> TTFTTRDGTQIYYKDWGSGQPIVFSHGWPLNADSWESQMIFLAAQGYRVIAHDRRGHGRSSQPWSGNDMDTYADDLAQLIEHLDLRDAVLFGFSTGGGEVARYIGRHG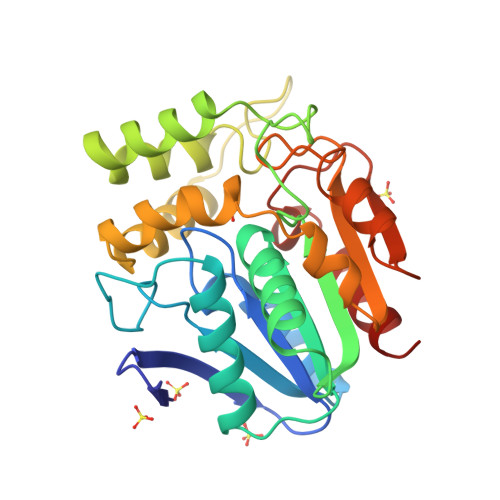TARVAKAGLISAVPPLMLKTEANPGGLPMEVFDGIRQASLADRSQLYKDLASGPFFGFNQPGAKSSAGMVDWFWLQGMAAGHKNAYDCIKAFSETDFTEDLKKIDVPTLVVHGDADQVVPIEASGIASAALVKGSTLKIYSGAPHGLTDTHKDQLNADLLAFIKG> SEVEYRAE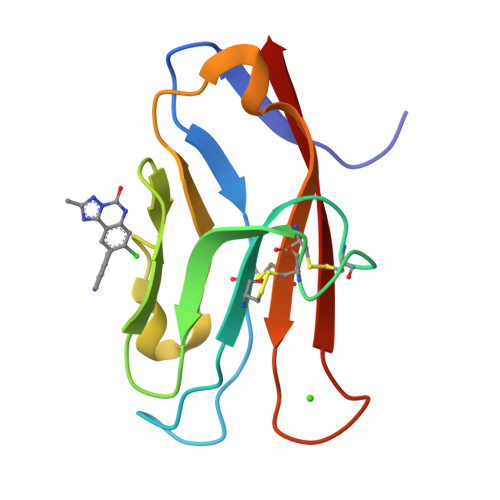VGQNAYLPCFYTPAAPGNLVPVCWGKGACPVFECGNVVLRTDERDVNYWTSRYWLNGDFRKGDVSLTIENVTLADSGIYCCRIQIPGIMNDEKFNLKLVIK>[44x]MNIMDFNVKKLAADAGTFLSRAVQFTEEKLGQAEKTELDAHLENLLSKAECTKIWTEKIMKQTEVLLQPNPNAR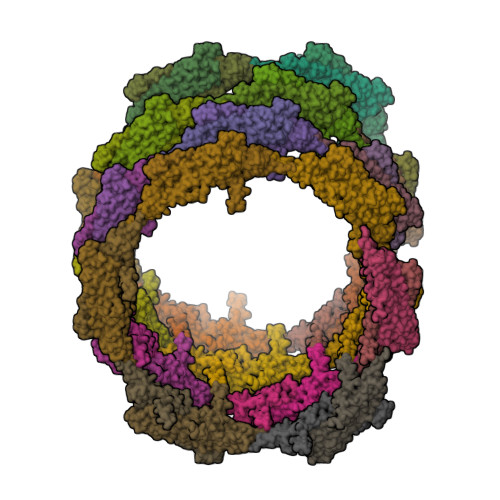IEEFVYEKLDRKAPSRINNPELLGQYMIDAGTEFGPGTAYGNALIKCGETQKRIGTADRELIQTSALNFLTPLRNFIEGDYKTIAKERKLLQNKRLDLDAAKTRLKKAKAAETRNSSEQELRITQSEFDRQAEITRLLLEGISSTHAHHLRCLNDFVEAQMTYYAQCYQYMLDLQKQLGSFPSNYLSNNNQTSVTPVPSVLPNAIGSSAMASTSGLVITSPSNLSDLKECSGSRKARVLYDYDAANSTELSLLADEVITVFSVVGMDSDWLMGERGNQKGKVPITYLELLN>[4x]APEGYRKLLDVQIFKDSPVVGWSGSGMGELETI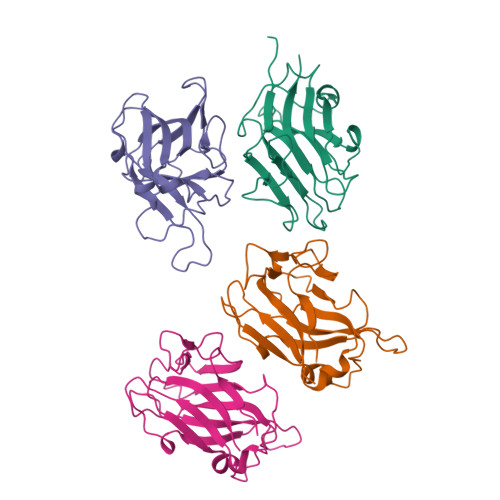GDTLPVDTTVTYNGLPTLRLNVQTTVQSGWWISLLTLRGWNTHDLSQYVENGYLEFDIKGKEGGEDFVIGFRDKVYERVYGLEIDVTTVISNYVTVTTDWQHVKIPLRDLMKINNGFDPSSVTCLVFSKRYADPFTVWFSDIKITSEDNEKSAPAIKVNQLGFIPEAEKYAL> MADYKDDDDKSGPDEVDASGRMGFVRQIQLLLWKNWTLRKRQKIRFVVELVWPLSLFLVLIWLRNANPLYSHHECHFPNKAMPSAGMLPWLQGIFCNVNNPCFQSPTPGESPGIVSNYNNSILARVYRDFQELLMNAPESQHLGRIWTELHILSQFMDTLRTHPERIAGRGIRIRDILKDEETLTLFLIKNIGLSDSVVYLLINSQVRPEQFAHGVPDLALKDIACSEALLERFIIFSQRRGAKTVRYALCSLSQGTLQWIEDTLYANVDFFKLFRVLPTLLDSRSQGINLRSWGGILSDMSPRIQEFIHRPSMQDLLWVTRPLMQNGGPETFTKLMGILSDLLCGYPEGGGSRVLSFNWYEDNNYKAFLGIDSTRKDPIYSYDRRTTSFCNALIQSLESNPLTKIAWRAAKPLLMGKILYTPDSPAARRILKNANSTFEELEHVRKLVKAWEEVGPQIWYFFDNSTQMNMIRDTLGNPTVKDFLNRQLGEEGITAEAILNFLYKGPRESQADDMANFDWRDIFNITDRTLRLVNQYLECLVLDKFESYNDETQLTQRALSLLEENMFWAGVVFPDMYPWTSSLPPHVKYKIRMDIDVVEKTNKIKDRYWDSGPRADPVEDFRYIWGGFAYLQDMVEQGITRSQVQAEAPVGIYLQQMPYPCFVDDSFMIILNRCFPIFMVLAWIYSVSMTVKSIVLEKELRLKETLKNQGVSNAVIWCTWFLDSFSIMSMSIFLLTIFIMHGRILHYSDPFILFLFLLAFSTATIMLCFLLSTFFSKASLAAACSGVIYFTLYLPHILCFAWQDRMTAELKKAVSLLSPVAFGFGTEYLVRFEEQGLGLQWSNIGNSPTEGDEFSFLLSMQMMLLDAAVYGLLAWYLDQVFPGDYGTPLPWYFLLQESYWLGGEGCSTREERALEKTEPLTEETEDPEHPEGIHDSFFEREHPGWVPGVCVKNLVKIFEPCGRPAVDRLNITFYENQITAFLGHNGAGKTTTLSILTGLLPPTSGTVLVGGRDIETSLDAVRQSLGMCPQHNILFHHLTVAEHMLFYAQLKGKSQEEAQLEMEAMLEDTG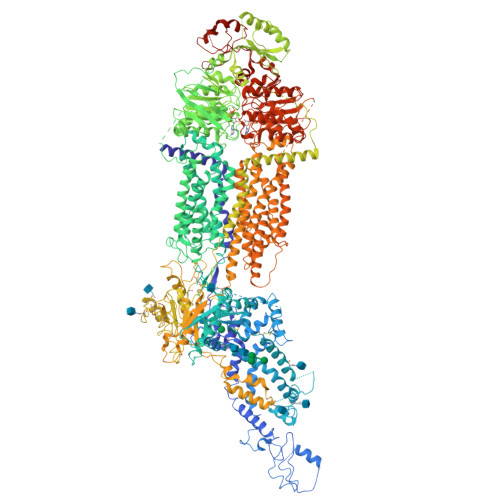LHHKRNEEAQDLSGGMQRKLSVAIAFVGDAKVVILDQPTSGVDPYSRRSIWDLLLKYRSGRTIIMSTHHMDEADLLGDRIAIIAQGRLYCSGTPLFLKNCFGTGLYLTLVRKMKNIQSQRKGSEGTCSCSSKGFSTTCPAHVDDLTPEQVLDGDVNELMDVVLHHVPEAKLVECIGQELIFLLPNKNFKHRAYASLFRELEETLADLGLSSFGISDTPLEEIFLKVTEDSDSGPLFAGGAQQKRENVNPRHPCLGPREKAGQTPQDSNVCSPGAPAAHPEGQPPPEPECPGPQLNTGTQLVLQHVQALLVKRFQHTIRSHKDFLAQIVLPATFVFLALMLSIVIPPFGEYPALTLHPWIYGQQYTFFSMDEPGSEQFTVLADVLLNKPGFGNRCLKEGWLPEYPCGNSTPWKTPSVSPNITQLFQKQKWTQVNPSPSCRCSTREKLTMLPECPEGAGGLPPPQRTQRSTEILQDLTDRNISDFLVKTYPALIRSSLKSKFWVNEQRYGGISIGGKLPVVPITGEALVGFLSDLGRIMNVSGGPITREASKEIPDFLKHLETEDNIKVWFNNKGWHALVSFLNVAHNAILRASLPKDRSPEEYGITVISQPLNLTKEQLSEITVLTTSVDAVVAICVIFSMSFVPASFVLYLIQERVNKSKHLQFISGVSPTTYWVTNFLWDIMNYSVSAGLVVGIFIGFQKKAYTSPENLPALVALLLLYGWAVIPMMYPASFLFDVPSTAYVALSCANLFIGINSSAITFILELFENNRTLLRFNAVLRKLLIVFPHFCLGRGLIDLALSQAVTDVYARFGEEHSANPFHWDLIGKNLFAMVVEGVVYFLLTLLVQRHFFLSQWIAEPTKEPIVDEDDDVAEERQRIITGGNKTDILRLHELTKIYPGTSSPAVDRLCVGVRPGECFGLLGVNGAGKTTTFKMLTGDTTVTSGDATVAGKSILTNISEVHQNMGYCPQFDAIDELLTGREHLYLYARLRGVPAEEIEKVANWSIKSLGLTVYADCLAGTYSGGNKRKLSTAIALIGCPPLVLLDQPTTGMDPQARRMLWNVIVSIIREGRAVVLTSHSMEECEALCTRLAIMVKGAFRCMGTIQHLKSKFGDGYIVTMKIKSPKDDLLPDLNPVEQFFQGNFPGSVQRERHYNMLQFQVSSSSLARIFQLLLSHKDSLLIEEYSVTQTTLDQVFVNFAKQQTESHDLPLHPRAAGASRQAQDLEGSDEVDAVEGSHHHHHHHHHH> IV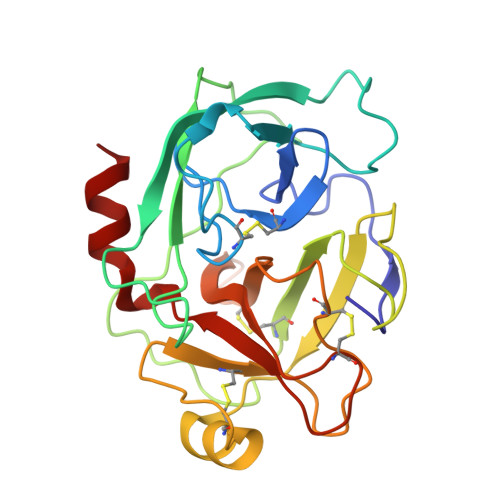GGSNAKEGAWPWVVGLYYGGRLLCGASLVSSDWLVSAAHCVYGRNLEPSKWTAILGLHMKSNLTSPQTVPRLIDEIVINPHYNRRRKDNDIAMMHLEFKVNYTDYIQPICLPEENQVFPPGRNCSIAGWGTVVYQGTTANILQEADVPLLSNERCQQQMPEYNITENMICAGYEEGGIDSCQGDSGGPLMCQENNRWFLAGVTSFGYKCALPNRPGVYARVSRFTEWIQSFLH> GQIKISKHANECGLPTIHTPSKTKLQPSVFYDVFPGSKEPAVLTDNDPRLKVNFKEALFSKYKGNTECSLNQHMEIAIAHYSAQLITLDIDSKPIALE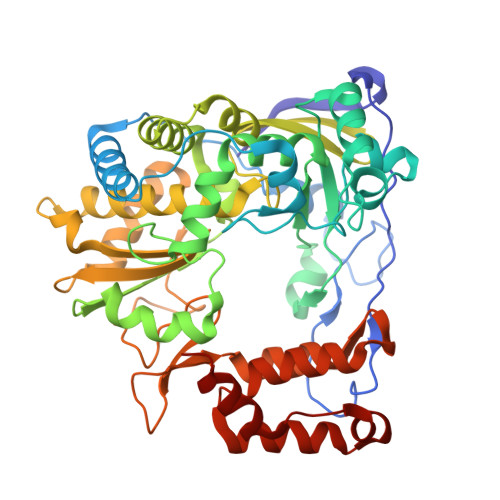DSVFGIEGLEALDLNTSAGFPYVTMGIKKRDLINNKTKDISRLKEALDKYGVDLPMITFLKDELRKKEKISAGKTRVIEASSINDTILFRTTFGNLFSKFHLNPGVVTGSAVGCDPETFWSKIPVMLDGDCIMAFDYTNYDGSIHPVWFQALKKVLENLSFQSNLIDRLCYSKHLFKSTYYEVAGGVPSGCSGTSIFNTMINNIIIRTLVLDAYKNIDLDKLKIIAYGDDVIFSYKYTLDMEAIANEGKKYGLTITPADKSTEFKKLDYNNVTFLKRGFKQDEKHTFLIHPTFPVEEIYESIRWTKKPSQMQEHVLSLCHLMWHNGRKVYEDFSSKIRSVSAGRALYIPPYDLLKHEWYEKF>SMQSSKRSSRSVEDDKEGHLVCRIGDWLQERYEIVGNLGEGTFGKVVECLDHARGKSQVALKIIRNVGKYREAARLEINVLKKIKEKDKENKFLCVLMSDWFNFHGHMCIAFELLGKNTFEFLKENNFQPYPLPHVRHMAYQLCHALRFLHENQLTHTDLKPENILFVNSEFETLYNEHKSCEEKSVKNTSIRVADFGSATFDHEHHTTIVATRHYRPPEVILELGWAQPCDVWSIGCILFEYYRGFTLFQTHENREHLVMMEKILGPIPSHMIHRTRKQKYFYKGGLVWDENSSDGRYVKENCKPLKSYMLQDSLEHVQLFDLMRRMLEFDPAQRITLAEALLHPFFAGLTPEERSFHT[2x]

The protein kinase CLK1 (cdc2-like kinase1) modulates activity of SPF45 by regulating its expression and by phosphorylating the protein at distinct serine residues. The CLK protein kinase family is closely related both in structure and function to the family of dual-specificity tyrosine phosphorylation-regulated kinases (DYRKs). The ATP binding pockets of CLK1 and DYRK1A are rather similar both in terms of sequence and surface shape. 3-Aryl-substituted 6,7-dihydropyrrolo[3,4-g]indol-8(1H)-ones were identified as inhibitors of the CLK protein kinase family.

While the 3-substituted derivative 8a was identified as a slightly selective inhibitor of CLK1, some 2,3-disubstituted congeners and a 6-oxo derivative were less active or not as selective versus casein kinase 1 (CK1) and against DYRKs. The X-ray structure analysis revealed that the inhibitor is localized in the ATP binding pocket, occupying a position similar to the binding mode predicted by the docking study for the pose in CLK1. As observed in the 8g/CLK1 complex, the lactam element of 8a establishes hydrogen bonds to the gk+1 and the gk+3 amino acids of CLK3, and the indole nitrogen forms a water-mediated hydrogen-bond to the hinge region. Compared to the situation of 8g in CLK1, 8a is slightly rotated in the binding pocket of CLK3 so that the indole nitrogen is veered away from the hinge region and the phenyl substituent is shifted slightly towards the DFG motif. The cavity near the αC-helix and the DFG motif is not occupied by the ligand, but by an ethylene glycol molecule which is kept in place by hydrogen bonds to the canonical Lys186 and Asp320 of the DFG motif. In further inhibitor design approaches this region of the binding pocket could be addressed by tailored side chains sprouting from the core element of new ligands. In contrast, all congeners showed considerably weaker or lacking inhibition of CLK3.1-(5-phenylpyridin-3-yl)-1,4-diazepane 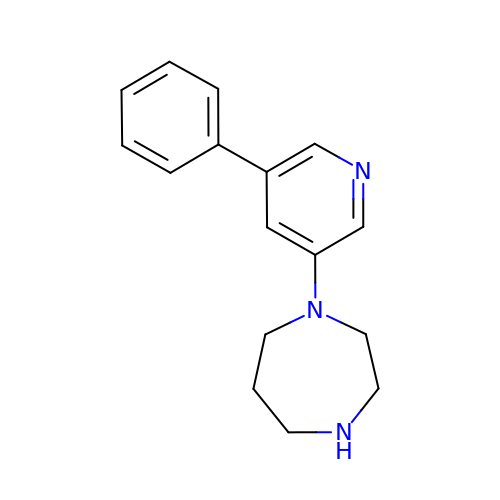| C16 H19 N3 | YAWZOEAWIFAGIV-UHFFFAOYSA-N> GNQGGFGNSRGGGAGLGNNQGSNMGGGMNF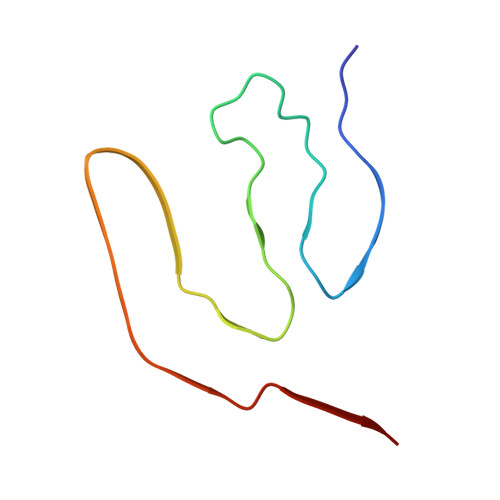GAFSINPAMMAAAQAALQSSWGMMGMLASQQN>GSRKDFIDTMTRELYDAFLHERLYLIYMDSRAE[2x];>[2x]MTMDTAQLKSQIQQYLVESGNYELISNELKARLLQEGWVDKVKDLTKSEMNINESTNFTQILSTVEPKALEMVSDSTRETVLKQIREFLEEIVDTQ;>GSPKKDKESIVLPTVGFDFIKDNETPSKKTSPKATS[4x]

In budding yeast, the TREX2 complex binds to NPCs and is thought to function in integrating the nuclear export of mature transcripts with earlier steps in the gene expression pathway, together with promoting genome stability through inhibiting R-loop formation (1–4). TREX2 is constructed from a Sac3 scaffold to which Thp1, Sem1, Cdc31 and two Sus1 chains bind. Sus1 and Cdc31 bind to the Sac3 centrin binding (CID) region (Sac3CID, residues 723–805) that has an unusually long α-helix about which the other three chains coil. We report here the crystal structure of the interface between TREX2 and Nup1 that shows that Nup1 residues 330–340 bind primarily to a cavity formed between the Sac3 helix (residues 757–777) and the Sus1 chain closest to Cdc31 (Sus1B) and show that Phe336Nup1 and Phe338Nup1 are crucial for this interaction.

Crystals with P3221 symmetry that diffracted to 3.0 Å resolution were obtained from a solution containing Nup1322–355 and Sac3757–787:Sus1B and crystals with P21 symmetry that diffracted to 2.6Å resolution were obtained with Nup1316–340 and the Sac3753–805:Sus1B:Cdc31 complex. Molecular replacement using appropriate search models derived from the Sac3CID domain complex showed clear difference density due to the Nup1 fragment, with the side chains of Phe336 and Phe338 being especially clear. For the P3221 crystals, Nup1 residues 326–340 were easily built into the difference density, albeit the Nup1 chains crossed from one Sac3:Sus1 complex in the asymmetric unit to the other in a form of domain swapping. Overall, the density of Nup1 residues 334–340 was much clearer than the remainder, consistent with residues 326–333 being bound more weakly. After iterative cycles of refinement and rebuilding, a final 2Fo-Fc map with excellent clarity was obtained. Density that could be assigned to residues 341–355 was absent from the final 2Fo-Fc and Fo-Fc maps. Vague density was visible in the place assigned to Nup1 residues 326–331 in the P21 crystal and it appears that in both crystals an additional Nup1 peptide chain became bound at this site. In both cases, the density due to this additional peptide chain was poor, consistent with it being bound weakly and/or sub-stoichiometrically and is likely the result of the peptide being present in molar excess during crystallogenesis, indicating that the binding of this second Nup1 chain was likely a crystallisation artefact. In the final model of both complexes, the structural arrangement of Sus1B bound to Sac3 and Cdc31 bound to Sac3 was essentially unaltered from that observed in the absence of Nup1 (17), consistent with Nup1 binding not generating a substantial conformational change. In both crystals, the principal Nup1 binding site was based on a cavity formed by Sus1B helices α1 and α2 and residues 757–787 of the Sac3CID domain helix.> GSHMVFRMELKIKHPLSKKDVKEIIAQLSQMFGEEIARKMLNKKDEVKV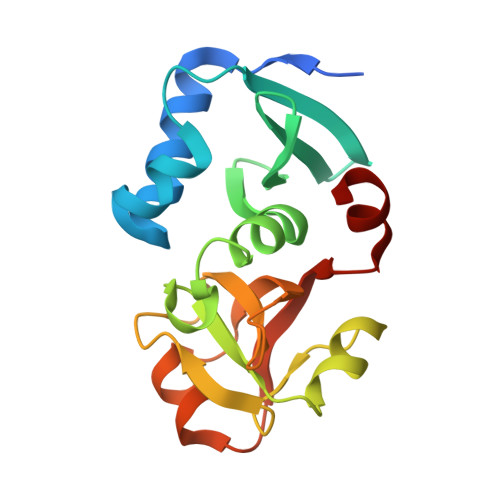AEFDKTTEIILVNDKPMFIRRKDLIFPLVIALYNLSDEEDLRKWPRRVVVDEGAVPHILNGADVMAPGIVDADEGIKEGDFVFVVEEKYGRPLAIGIALMSGKVMKEKNRGKAVKVIHHARDKIWEVTAR> GSHMNRDILRTLSLKGDHNIRVAILDGPVDIAHPCFQGADL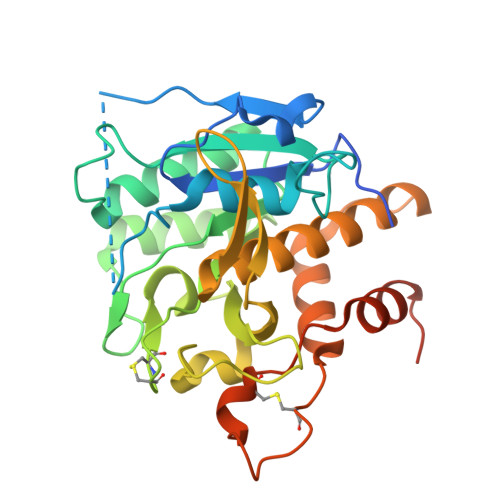TVLPTLAPTAARSDGFMSAHGTHVASIIFGQPETSVPGIAPQCRGLIVPIFSDDRRRITQLDLARGIERAVNAGAHIINISGGELTDFGEADGWLENAVSLCRQNNVLLVAAAGNNGCDCLHVPAALPAVLAVGAMDDHGHPLDFSNWGSTYEQQGILAPGEDILGAKPGGGTERLSGTSFATPIVSGVAALLLSEQVRRGETPDPQKVRQLLLQSALPCDDDAPEQARRCLAGRLNVSGAFTLLKGGNMSEELATASFPSVEAS> PISPIETVPVKLKPGMDGPKVKQWPLTEEKIKALVEICTEMEKEGKISKIGPENPYNTPVFAIKKKDSTKWRKLVDFRELNKRTQDFWEVQLGIPHPAGLKKKKSVTVLDVGDAYFSVPLDEDFRKYTAFTIPSINNETPGIRYQYNVLPQGWKGSPAIFQSSMTKILEPFKKQNPDIVIYQYMDDLYVGSDLEIGQHRTKIEELRQHLLRWGLTTPD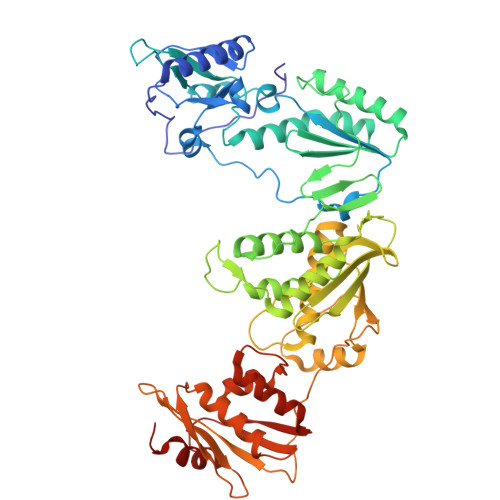KKHQKEPPFLWMGYELHPDKWTVQPIVLPEKDSWTVNDIQKLVGKLNWASQIYPGIKVRQLCKLLRGTKALTEVIPLTEEAELELAENREILKEPVHGVYYDPSKDLIAEIQKQGQGQWTYQIYQEPFKNLKTGKYARMRGAHTNDVKQLTEAVQKITTESIVIWGKTPKFKLPIQKETWETWWTEYWQATWIPEWEFVNTPPLVKLWYQLEKEPIVGAETFYVDGAANRETKLGKAGYVTNKGRQKVVPLTNTTNQKTQLQAIYLALQDSGLEVNIVTDSQYALGIIQAQPDKSESELVNQIIEQLIKKEKVYLAWVPAHKGIGGNEQVDKLVSAGIRKIL(1R)-3-amino-1-[3-(cyclohexylmethoxy)-4-fluorophenyl]propan-1-ol 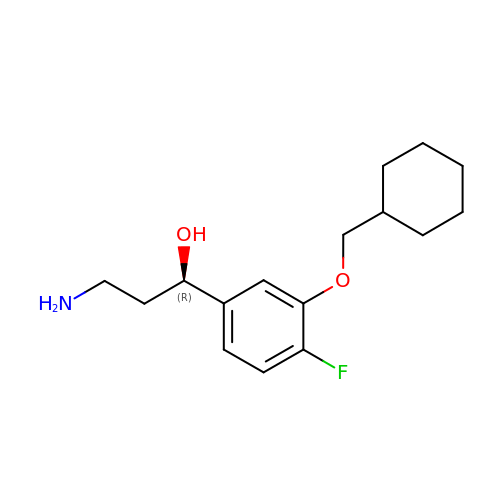| C16 H24 F N O2 | CYDVSJHNBXQOGZ-OAHLLOKOSA-N>SMMSSLDINEQRALIKSAHRYISEKLEDHFSSEFLPKALVICGEGLSGISTKIADEPKPLILSYSTIPGFKVSTVPGHSGELIFGYMNGAPVVLMNGRLHSYEGHSLAETVHPIRALHLLGSINVL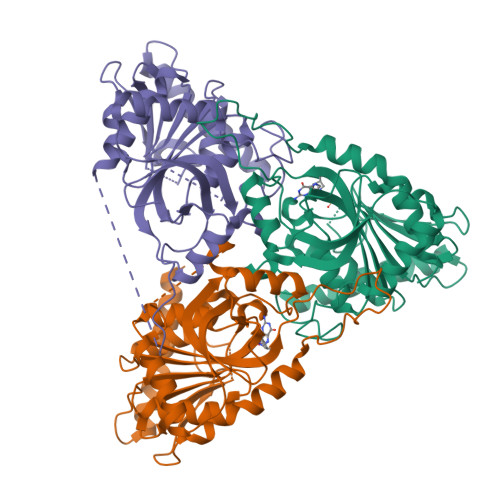IVTNAAGGINASFKAGDLMCVYDHINFPGLCGFHPLRGANFDEFGPRFLATSDAYDLELRKLLFSKKKELNIERKIHEGTYSYVHGPTFESRAESRFLRLAGTDAVGMSTVPEVVTARHCGWRVLALSLITNECVVDPPASAHDENPVPIQEGKATHEEVLENSAKASKDVQELIFSVVAEI[6x]> MANEEDDPVVQEIDVYLAKSLAEKLYLFQYPVRPASMTYDDIPHLSAKIKPKQQKVELEMAIDTLNPNYCRSKGEQIALNVDGACADETSTYSSKLMDKQTFCSSQTTSNTSRYAAALYRQGELHLTPLHGILQLRPSFSYLDKADAKHREREAANEAGDSSQDEAEDDVKQITVRFSRPESEQARQRRVQSYEFLQKKHAEEPWVHLHYYGLRDSRSEHERQYLLCPGSSGVENTELVKSPSEYLMMLMPPSQEEEKDKPVAPSNVLSMAQLRTLPLADQIKILMKNVKVMPFANLMSLLGPSIDSVAVLRGIQKVAMLVQGNWVVKSDILYPKDSSSPHSGVPAEVLCRGRDFVMWKFTQSRWVVRKEVATVTKLCAEDVKDFLEHMAVVRINKGWEFILPYDGEFIKKHPDVVQRQHMLWTGIQAKLEKVYNLVKETMPKKPDAQSGPAGLVCGDQRIQVAKTKAQQNHALLERELQRRKEQLRVPAVPPGVRIKEEPVSEEGEEDEEQEAEEEPMDTSPSGLHSKLANGLPLGRAAGTDSFNGHPPQGCASTPVARELKAFVEATFQRQFVLTLSELKRLFNLHLASLPPGHTLFSGISDRMLQDTVLAAGCKQILVPFPPQTAASPDEQKVFALWESGDMSDQHRQVLLEIFSKNYRVRRNMIQSRLTQECGEDLSKQEVDKVLKDCCVSYGGMWYLKGTVQS

Pol III is a multi-subunit complex composed of 17 subunits. The TFIIF-like RPC4/5 and the TFIIE-like RPC3/6/7 subcomplexes are Pol III specific and can be regarded as built-in general transcription factors that play a fundamental role in Pol III transcription initiation and termination. A notable exception is the subunit RPC5, which in metazoans encompasses a long C-terminal extension (RPC5EXT, ~450 residues long), whose function is currently unknown. The RPC5EXT is formed by two consecutive tandem winged helix domains (tWHD1 residues 259–440; tWHD2 residues 556–708) connected by a 115 residue-long flexible linker.

To gain insight into the structure and function of RPC5EXT, we determined the structure of its individual domains by X-ray crystallography. Of the two tWHDs, tWHD1 is the most conserved while tWHD2 is absent in Caenorhabditis elegans and Drosophila melanogaster. The tWHD1 is formed by two juxtaposed winged helix domains that form a compact globular domain with one of the two recognition helices, typically involved in DNA binding, buried within the structure. The compact conformation of tWHD1 is observed also in solution as highlighted by small-angle X-ray scattering (SAXS) data. Thus, one possibility is that, analogously to A49 tWHD, the RPC5-tWHD1 participates in an interaction with the upstream DNA and bound transcription factors, thus stabilizing the human Pol III PIC.>[2x]MEILDRPQAPSDFNPMSEQSFRDPASICQRAREETPVFFYAPLGVWMVTRREDAERVLSEWETFSSLANSPNVPEEFRSRFAPSVMADSIVAIDPPRHTQARNVIQRGFMKPKIDPLEPIIEQRAHEIIDRFAGESGTEIMNNYCLELTTRTLMALYDLPLEDRPMFERIRDVSIKVLASVYEPMQEPEKSRVWNEYVSGYEYFYQLVEQRRNSDARDIISTMASQKDNQGNPALSTERI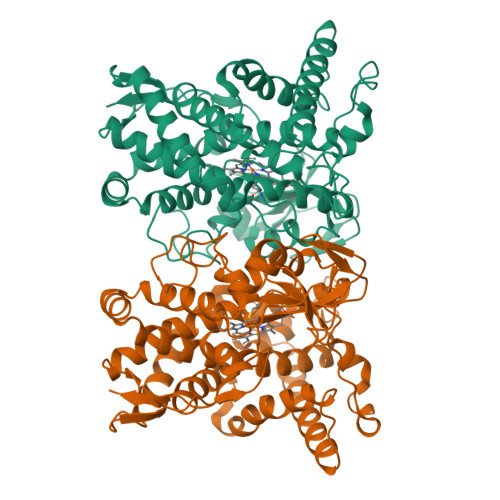ALHLVEIAFAGTDTTAQMMANAILFLDSHPEALAAAKADKTLWSRVFEETVRRRPSAPFAGRITTTEVEIQGVKIPAGSPVWVSLAAANTDPRHVGCPMNFDINREAPQDHLAFTKGRHTCPGAPLARLQGATGLRVLFERLPELKVVPDQPLNFAPMALLPVRLSLQVIW>[14x]AEPVYPDQLRLFSLGQGVCGDKYRPVNREEAQSVKSNIVGMMGQWQISGLANGWVIMGPGYNGEIKPGTASNTWCYPTNPVTGEIPTLSALDIPDGDEVDVQWRLVHDSANFIKPTSYLAHYLGYAWVGGNHSQYVGEDMDVTRDG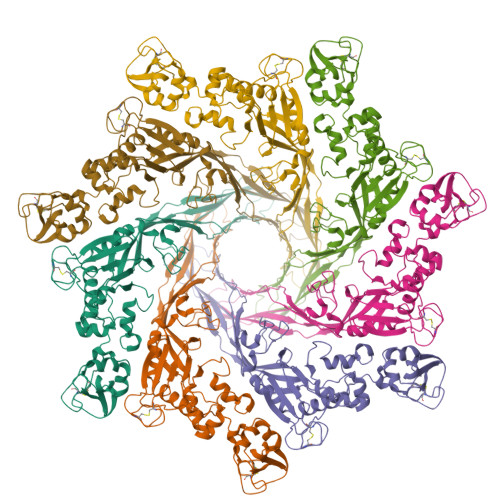DGWVIRGNNDGGCDGYRCGDKTAIKVSNFAYNLDPDSFKHGDVTQSDRQLVKTVVGWAVNDSDTPQSGYDVTLRGDTATNWSKTNTYGLSEKVTTKNKFKWPLVGETELSIEIAANQSWASQNGGSTTTSLSQSVRPTVPARSKIPVKIELYKADISYPYEFKADVSYDLTLSGFLRWGGNAWYTHPDNRPNWNHTFVIGPYKDKASSIRYQWDKRYIPGEVKWWDWNWTIQQNGLSTMQNNLARVLRPVRAGITGDFSAESQFAGNIEIGAPVPLAA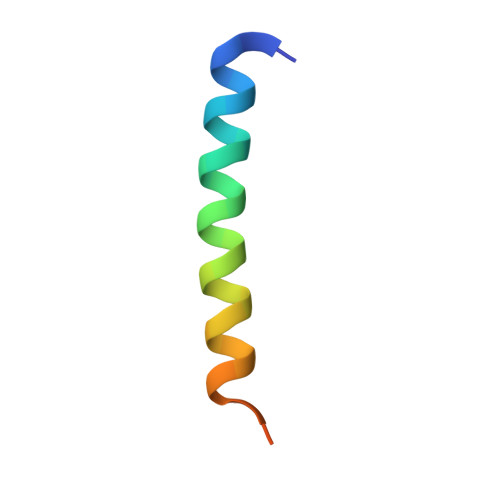> GPSWARQESLQERKQALYEYARRRFTERRAQEAD({3-[1-(4-HYDROXY-2-OXO-2H-CHROMEN-3-YL)-PROPYL]-PHENYLCARBAMOYL}-METHYL)-CARBAMIC ACID TERT-BUTYL ESTER 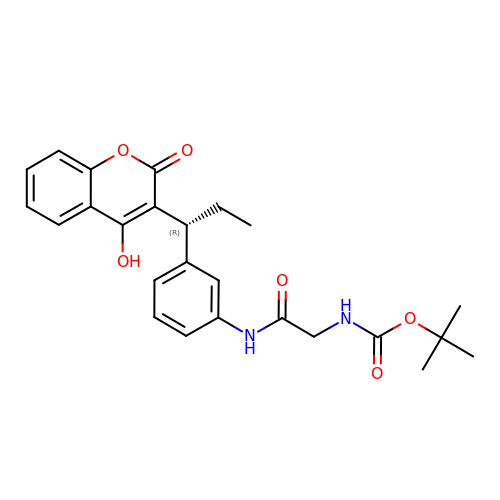| C25 H28 N2 O6 | QUQQVMVIWCUYFV-KRWDZBQOSA-N>[2x]MTMASVPASRYLTDMTLEEMSRDWSM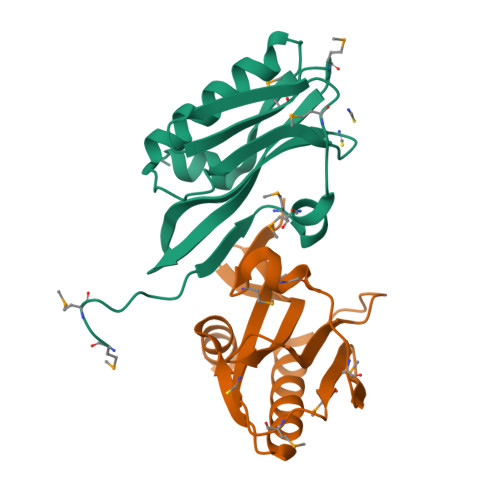LIPKQKVAGPLCIRMDQAIMDKNIILKANFSVIFDRLETLILLRAFTEEGAIVGEISPLPSLPGHTAEDVKNAVGVLIGGLEWNDNTVRVSETLQRFAWRSSN Clusterin (apolipoprotein J), a conserved glycoprotein abundant in blood and cerebrospinal fluid, functions as a molecular chaperone and apolipoprotein. The Clu structure is composed of three domains, a coiled-coil (CC) domain, a small helical domain containing all disulfide bridges (hereafter disulfide domain, DD) and a C-terminal α/β roll-like (AB) domain. Structure-based mutational analysis demonstrated that two disordered, hydrophobic peptide tails enable diverse activities. Resembling the substrate-binding regions of small heat-shock proteins, these sequences mediate clusterin’s chaperone function in suppressing amyloid-β, tau and α-synuclein aggregation.

For crystallization, we designed a single-chain construct (Clu-Δ(214–238)) comprising a deletion of a predicted unstructured sequence including the furin cleavage site. Upon expression in the presence of the α-mannosidase I inhibitor kifunensine to generate uniform oligomannose N-glycans, purified Clu-Δ(214–238) crystallized at acidic pH in two distinct lattice types, crystal forms I and II, diffracting to 2.8-Å and 3.5-Å resolution, respectively. Crystal form I contained one copy of Clu-Δ(214–238) while crystal form II contained two independent copies. aData from two crystals were merged for processing of crystal form II. The three conformations in the crystal lattices differed slightly in their domain orientations, with root-mean-square deviation (r.m.s.d.) values of 1.5–2.0 Å (Cα positions). While the DD seems fairly rigid, its linkers to helices α2 and α10 deviate considerably between crystal forms, indicating structural plasticity. The N-glycans in Clu-Δ(214–238) point toward solvent channels in the crystal lattices and are partially ordered (gray spheres). Importantly, the model of the WT structure contains extended unstructured regions, including disordered tails at the C terminus of the β-chain (residues 199–227) and at the N terminus of the α-chain (residues 228–244). These tails are generated by furin cleavage in the unstructured sequence of WT Clu that is deleted in Clu-Δ(214–238).

>[2x]DQTVSDNELQEMSNQGSKYVNKEIQNAVNGVKQIKTLIEKTNEERKTLLSNLEEAKKKKEDALNETRESETKLKELPGVCNETMMALWEECKPCLKQTCMKFYARVCRSGSGLVGRQLEEFLNQSSPFYFWMNGDRIDSLLENDRQQTHMLDVMQDHFSRASSIIDELFQDRFFTREPQDTYHYLPFSLPHNFHAMFQPFLEMIHEAQQAMDIHFHSPAFQHPPTEFIREGDDDRTVCREIRHNSTGCLRMKDQCDKCREILSVDCSTNNPSQAKLRRELDESLQVAERLTRKYNELLKSYQWKMLNTSSLLEQLNEQFNWVSRLANLTQGEDQYYLRVTTVASHTSDSDVPSGVTEVVVKLFDSDPITVTVPVEVSRKNPKFMETVAEKALQEYRKKHREE>[6x]MFYINSKYKIDLDKIMTKMKNKSVINIDDVDDEELLAILYTSKQFEKILKNNEDSKYLENKVFCSVFLEPSTRTRCSFDAAILKLGSKVLNITDMNSTSFYKGETVEDAFKILSTYVDGIIYRDPSKKNVDIAVSSSSKPIINAGNGTGEHPTQSLLDFYTIHNYFPFILDRNINKKLNIAFVGDLKNGRTVHSLSKLLSRYNVSFNFVSCKSLNIPKDIVNTITYNLKKNNFYSDDSIKYFDNLEEGLEDVHIIYMTRIQKERFTDVDEYNQYKNAFILSNKTLENTRDDTKILHPLPRVNEIKVEVDSNPKSVYFTQAENGLYVRMALLYLIFSSTSSAWSHPQFEK

Aspartate transcarbamoylase (ATC) catalyzes the second step of de novo pyrimidine synthesis, combining l-aspartate (l-ASP) and carbamoyl phosphate (CP) to form carbamoyl-aspartate (CP-ASP) and phosphate. Aspartate transcarbamoylase (ATC) has been suggested to be a promising target for antimalarial drug development. In depth structural analysis of the ATC catalytic cycle has been performed previously, which indicated that ATC exists in a low substrate affinity “T” state and a high substrate affinity “R” state. Here, we describe a series of small-molecule inhibitors of P. falciparum ATC with low nanomolar binding affinities that selectively bind to a previously unreported allosteric pocket, thereby inhibiting ATC activation.

BDA-04 shows strong selectivity, with measured IC50s of 77.2 nM and 2.8 μM against PfATC and HsATC, respectively. To further characterize BDA-04, we then performed microscale thermophoresis (MST) that determined the Kd of BDA-04 as 66.3 nM. To characterize the mechanism of inhibition by BDAs, enzyme activity assays were performed using BDA-04 as an exemplar. This analysis indicates that BDA-04 acts as a noncompetitive inhibitor with CP and Asp. The structure demonstrated BDA-04 bound to the allosteric pocket shielded from the solvent by the 120 s loop and extending into the channel to the active site. The terminal benzene side chain of BDA-04 is deeply buried in this hydrophobic area formed by the α3 helix, α4 helix, and β1–3 sheets from an adjacent subunit. The 5-phenylthiophene ring extends from the hydrophobic binding site to the “gate” of the pocket, blocking access to the allosteric pocket. The Boc moiety of BDA-04 partially occludes the CP binding domain. However, in the BDA-04:PfATC complex, Ser135 and Lys138 shift out of the CP binding site as the 120 s loop is blocked by BDA-04. Binding of BDA-04 completely blocked the movement of the 120 s loop, with the amino groups of the gatekeepers Ser135 and Lys138 moving by 8.5 and 7.1 Å, compared to their active position, respectively. BDA-04 therefore inhibits PfATCase allosterically, by stabilizing PfATC in inactive state that indirectly blocks the binding and recognition of CP.(R)-N2-(4-(cyclopropylmethoxy)-3,5-difluorophenyl)-5-(3-methylpiperazin-1-yl)-N4-(tetrahydro-2H-pyran-4-yl)pyrimidine-2,4-diamine | C24 H32 F2 N6 O2 | 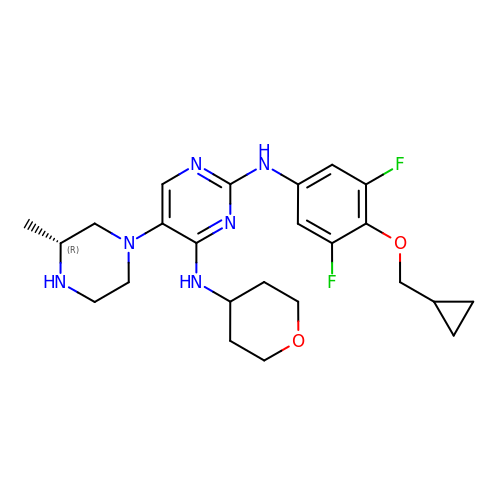FPYULJCYPOLXGV-OAHLLOKOSA-N> MTNIIQADEPTTLTTNALDLNSVLGKD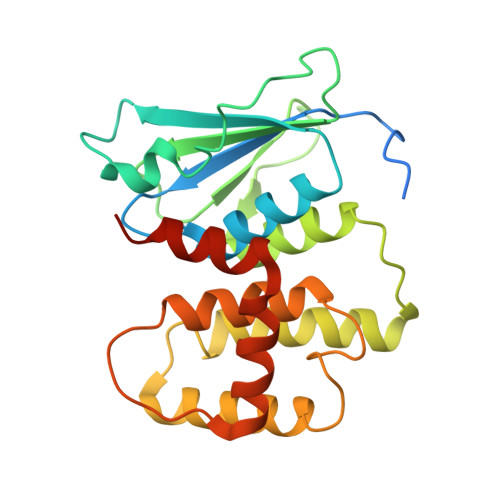YGALKDIVINANPASPPLSLLVLHRLLCEHFRVLSTVHTHSSVKSVPENLLKCFGEQNKKQPRQDYQLGFTLIWKNVPKTQMKFSIQTMCPIEGEGNIARFLFSLFGQKHNAVNATLIDSWVDIAIFQLKEGSSKEKAAVFRSMNSALGKSPWLAGNELTVADVVLWSVLQQIGGCSVTVPANVQRWMRSCENLAPFNTALKLLKLEHHHHHH>[2x]MAHPGRTGYDNREIVMKYIHYKLSQRGYEWDAGDDVEENRTEAPEGTESEVVHLTLRQAGDDFSRRYRRDFAEMSSQLHLTPFTARGRFATVVEELFRDGVNWGRI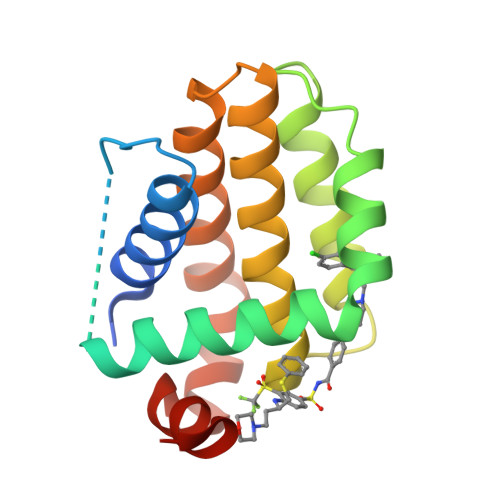VAFFEFGGVMCVESVNREMSPLVDNIALWMTEYLNRHLHTWIQDNGGWDAFVELYGPSMR>GAMAQNEQEQAEQTLEKPAEPVKLETIFVTAEEQVKQSLGVSVITKEDLEKLPVRNDISDYVRRMPGVNLTGNSATGQRGNNRQIDIRGMGPE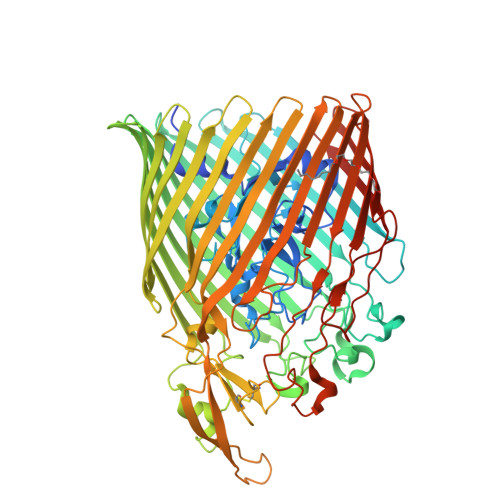NTLILVDGKPINSRNSVRYGWKGERDTRGDSNWVPAEAIESIEVLRGPAAARYGSGAAGGVVNIITKKVTNETHGSVEFYTSQPEDSKEGSSNRVGFNVSGPLIKDVLSYRLYGNYNKTEADDVDINKSIGSTAAGREGVKNKDISGRLAWQATDQQTVLLDISSSKQGNIYSGDSQLNANAEADAILSQLIGKETNTMYRDSYALTHEGDWSWGKSKLVAQYDKTHNKRLPEGLAGSVEGKINNLDDKATSRLETLRFNGEANIPFEYYLPQVLTVGTEWVEDRFKDNVSTTQGKDSSGSGYGDQLAKGDRSKMESRIASAYIEDNLKVTDSTDVVLGLRFDDHSKSGSNWSPSLNITQKLNDYFTLKGGVAKAYKAPNMYQNAEGYLLSTNGNGCPANIESRCLLQGNGDLKPETSVNKELGIQFQKDIVNASLTWFRNDYKDKIVAGTHVVGTVDGSSTNANTGAVTNTKWNILRWENTPKALIQGFEGSLGLDFGDIRWTNNFTYMMDSKDKQTGNPLSLVPIYTINSIFDYDITDQLDVNFVFTQYGRQKSRQFAENRLESGIGSGGANSALKPSTVKSYSTAGINVGYKFSDQISTRVGVSNLFDKQILRDSNSISQTYNEPGRAYYASLKYSF[2x]>SENVGKKYFMSSVRRMPLNRAKALCSELQGTVATPRNAEENRAIQNVAKDVAFLGITDQRTENVFEDLTGNRVR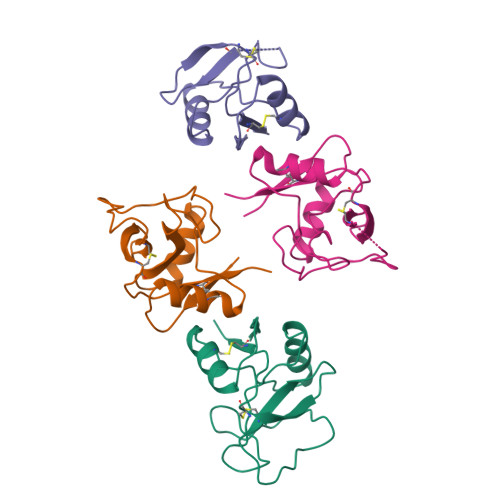YTNWNEGEPNNVGSGENCVVLLTNGKWNDVPCSDSFLVVCEFSD[4x]> MFEKFLERSGNSIKLE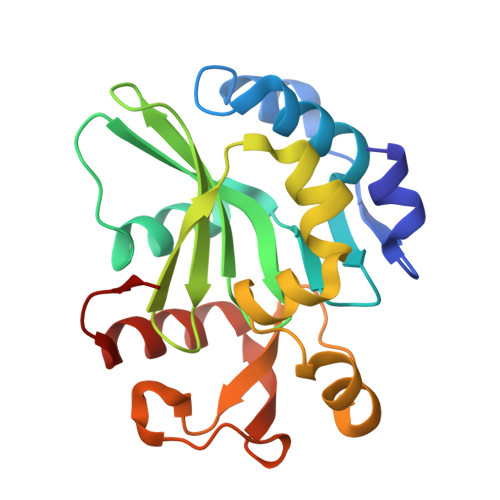EFSEDYIRQYNNLVSEKLISFWRIAGIGIYCNGLFRTIIPNDYQYIIEECYPMYDYETVTPFMITVFGDIFAYVKNHVIGDYVVFINIRYGTFKILSENIDILLNIVIFNKSCLENWFLLNEYNTIKEVKAMPKIDECYGYVPALVAGGKDCIDNIQIVKIAPYIDTVIQLMGDLKRIR> SLYKMSSINADFAFNLYRRFTVETPDKNIFFSPVSISAALVMLSFGACCSTQTEIVETLGFNLTDTPMVEIQHGFQHLICSLNFPKKEL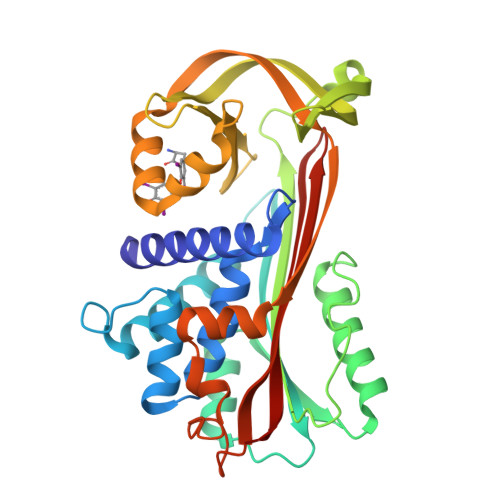ELQIGNALFIGKHLKPLAKFLNDVKTLYETEVFSTDFSNISAAKQEINSHVEMQTKGKVVGLIQDLKPNTIMVLVNYIHFKAQWANPFDPSKTEDSSSFLIDKTTTVQVPMMHQMEQYYHLVDMELNCTVLQMDYSKNALALFVLPKEGQMESVEAAMSSKTLKKWNRLLQKGWVDLFVPKFSISATYDLGATLLKMGIQHAYSENADFSGLTEDNGLKLSNAAHKAVLHIGEKGTEAAGAMFLEAIPR;> SENTFLHPIIQIDRSFMLLILERSTRSILFLGKVVNPTEA>HHHHHHSSGLVPRGSHMVVADTKSLKLLALADKVAKTDANVMILGPSGSGKEVMSRYIHNASPRKEGPFIAINCAAIPDNMLEATLFGYEKGAFTGAVQACPGKFEQAQGGTILLDEISEMDLNLQAKLLRVLQEREVERLGSRKSIKLDVRVLATSNRDLKQYVQAGHFREDLYYRLNVFPLTWPALCERKDDIEPLANHLIERHCKKLGLPVPSIAPNAITKLLNYPWPGNVRELDNVVQRALILSENGHIQSEH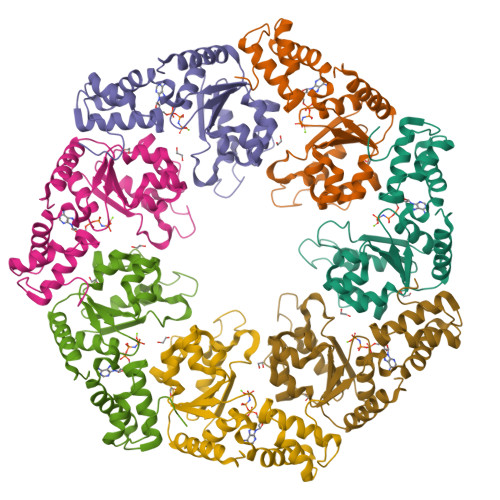ILLEGVDWHD[7x]> SKILVIAEHRRNDLRPVSLELIGAANGLKKSGEDKVVVAVIGSQADAFVPALSVNGVDELVVVKGSSIDFDPDVFEASVSALIAAH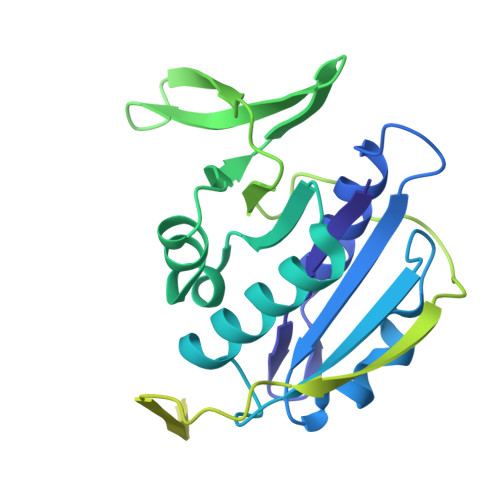NPSVVLLPHSVDSLGYASSLASKTGYGFATDVYIVEYQGDELVATRGGYNQKVNVEVDFPGKSTVVLTIRPSVFKPLEGAGSPVVSNVDAPSVQSRSQNKDYVEVGGGNDIDITTVDFIMSIGRGIGEETNVEQFRELADEAGATLCCSRPIADAGWLPKSRQVGQSGKVVGSCKLYVAMGISGSIQHMAGMKHVPTIIAVNTDPGASIFTIAKYGIVADIFDIEEELKAQLAA> PFNGDREAHPPFTLKGSVYNDPFIKDLEHRKEFIASGFNTNYAYERVLTEAFMGLGC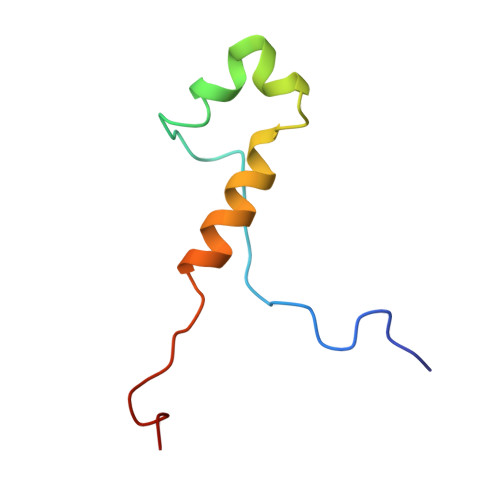VISEEL>[3x]GPASIASSFRKNAAGNFGPELARKLSQLVKTEKGVLRAMEVVASERREAAKQLSLWGADNDDDVSDV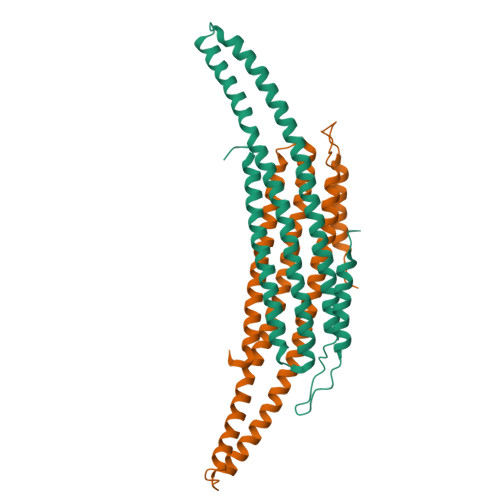TDKLGVLIYELGELQDQFIDKYDQYRVTLKSIRNIEASVQPSRDRKEKITDEIAHLKYKDPQSTKIPVLEQELVRAEAESLVAEAQLSNITREKLKAAYSYMFDSLRELSEKFALIAGYGKALLELLDDSPVTPGEARPAYDGYEASRQIIMDAESALESWTLDMAA> MSVGIVYGDQYRQLCCSSPKFGDRYALVMDLINAYKLIPELSRVPPLQWDSPSRMYEAVTAFHSTEYVDALKKLQMLHCEEKELTADDELLMDSFSLNYDCPGFPSVFDYSLAAVQGSLAAASALICRHCEVVINWGGGWHHAKRSEASGFCYLNDIVLAIHRLVSSTPPETSPNRQTRVLYVDLDLHHGDGVEEAFWYSPRVVTFSVHHASPGFFPGTGTWNMVDNDKLPIFLNGAGRGRFSAFNLPLEEGINDLD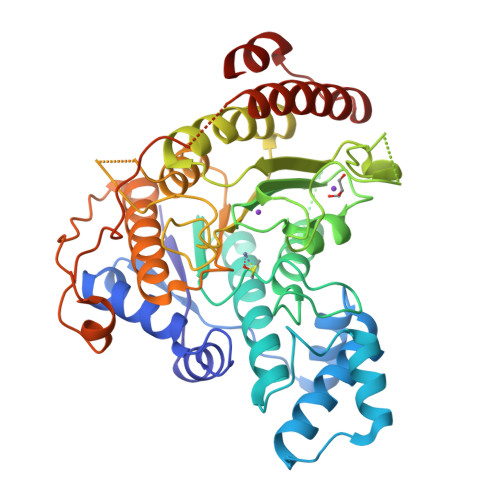WSNAIGPILDSLNIVIQPSYVVVQCGADCLATDPHRIFRLTNFYPNLNLDSDCDSECSLSGYLYAIKKILSWKVPTLILGGGGYNFPDTARLWTRVTALTIEEVKGKKMTISPEIPEHSYFSRYGPDFELDIDYFPHKSHNKTLDSIQKHHRRILEQLRNYADLNKLIYDYDQVYQLYNLTGM> HHHHHHSQDPMSNTADFRLQTSTLCHSFLLASANKQDTDYLTDLLDNTNIDLTCVPNGQ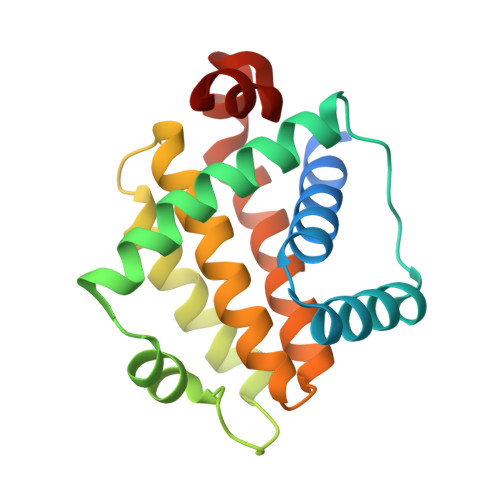EIIHSLLQLVGDFNQRFSQTHEIEPVAQSLGIDSDKPVDKTALEIFYLEILNGLFEKLNWGRIVAMFAFLRILVLRLSKHGHSDAIQMLIKTTSQYSDEKLKNWINLHDGWSGLIEFSGR> MTQFDKQYNSIIKDIINNGISDEEFDVRTKWDSDGTPAHTLSVISKQMRFDNSEVPILTTKKVAWKTAIKELLWIWQLKSNDVNDLNMMGVHIWDQWKQEDGTIGHAYGFQLGKKNRSLNGEKVDQVDYLLHQLKNNPSSRRHITMLWNPDELDAMALTPCVYETQWYVKHGKLHLEVRA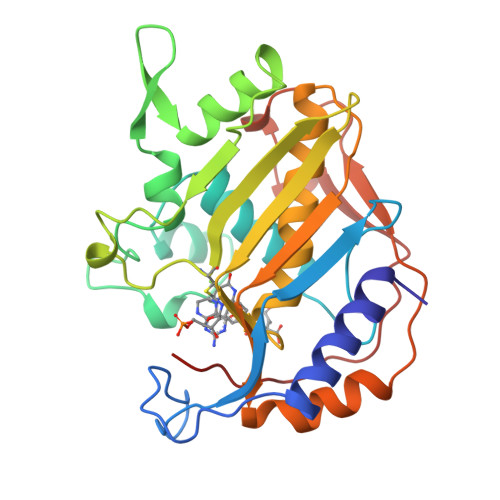RSNDMALGNPFNVFQYNVLQRMIAQVTGYELGEYIFNIGDCHVYTRHIDNLKIQMEREQFEAPELWINPEVKDFYDFTIDDFKLINYKHGDKLLFEVAV(2S)-2-[(2-azanyl-4-oxidanylidene-3H-pteridin-7-yl)carbonylamino]-3-phenyl-propanoic acid | 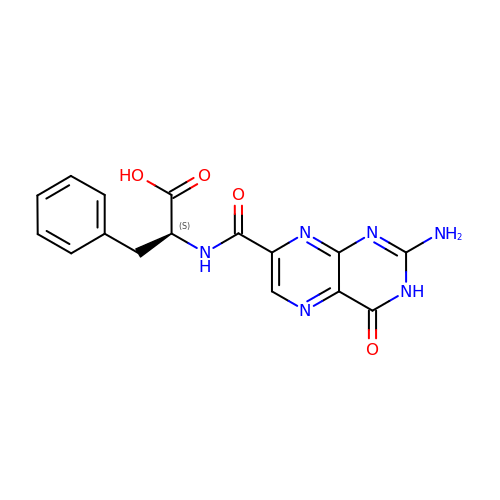C16 H14 N6 O4 | AJHMFJMLQDPCOX-VIFPVBQESA-N>[4x]SMQDPTIFEERHLKYISQLGKGNFGSVELCRYDPLGDNTGALVAVKQLQHSGPDQQRDFQREIQILKALHSDFIVKYRGVSYGPGRQSLRLVMEYLPSGCLRDFLQRHRARLDASRLLLYSSQICKGMEYLGSRRCVHRALAARNILVESEAHVKIADFGLAKLLPLDKDYYVVREPGQSPIFWYAPESLSDNIFSRQSDVWSFGVVLYELFTYCDKSCSPSAEFLRMMGSERDVPALSRLLELLEEGQRLPAPPACPAEVHELMKLCWAPSPQDRPSFSALGPQLDMLWSGSR

However, cysteines at the αD-1 position exist also in six other kinases, namely most members of the HER family (EGFR, HER2 and HER4), the Janus kinase JAK3, the SRC kinase BLK and the mitogen activated protein kinase kinase MKK7 (MAP2K7). Our previous study demonstrated the successful use of the tricyclic imidazo [5,4-d]pyrrolo[2,3-b]pyridine scaffold for the design of selective covalent-reversible JAK3 probes FM-381 (5a) and FM-409 (5b) targeting JAK3 C909 via an α-cyano acrylamide warhead. Based on this, we aimed to expand the inhibitor series and explore their potentials as irreversible inhibitors for JAK3 and other kinases that harbor a cysteine at the equivalent position. The determined crystal structures of 9a and 10a in complex with JAK3 confirmed the predicted hinge interaction pattern and covalent modification of C909.

We hypothesized that the 1H-pyrrolo[2,3-b]pyridine (7-azaindole) core in 9a might adopt an inverted binding orientation when compared to 5a,b or common 7H-pyrrolo[2,3-d]pyrimidine derived JAK inhibitors like 4 with two hydrogen bonds between the 7-azaindole and the backbone of L905. As expected, the 7-azaindole core in both compounds was anchored to the hinge region via two hydrogen bonds with the L905 backbone NH and carbonyl oxygen atom, respectively. The warhead amide was present in two flipped conformations and involved in water-mediated hydrogen bonds, most notably with the backbone of C909. The latter interactions may assist in pre-orienting the Michael acceptor to facilitate cysteine addition. To examine whether our replacement strategy of the hinge binding motif for expanding the profile of the JAK3 covalent inhibitors to other kinases succeeded, we characterized the activity of inhibitors 9a and 10a against all kinases featuring the αD-1 cysteine. This screening revealed that the compounds strongly inhibited BMX and TXK with no or less significant binding to other kinases at 200 nM.> GAMEPSAPKELKFGDITKDSVHLTWEPPDDDGGSPLTGYVVEKREVSRKTWTKVMDFVTDLEFTVPDLVQGKEYLFKVCARNKCGPGEPAYVDEPVNM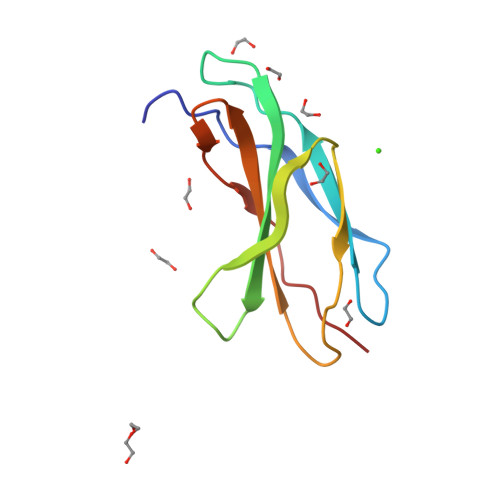S> KKKK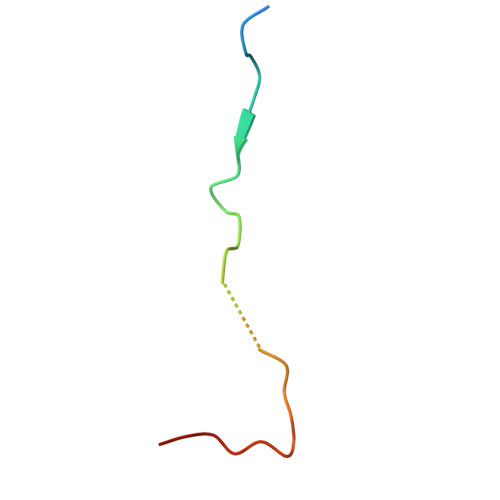REHACFENPGLNLELPEKQFNPYEVVRSA> G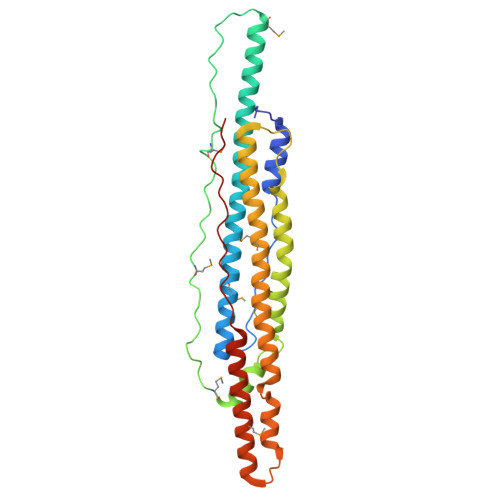SHMSEELQYELPGLERKAHECESTRPEGPGDATKPDELATTASVYSKLMASAAKLKATFAAGDREGERIAAAIRAAAGAYQKIEEQKAAELSRQMNGSDAPPPAAEAVVPDMSGIPGPLAIPSMEYPSAAAAADEMDWEAAARIIHSGDTQALSMKYFRDQWRDYQSTLEGHGRHFANPAEGWAGAAAETCAEAQRRLSTWWADMGAECGRLAQEATTFVDAHDKLVANHPTLENVREFEETEWASEWDRQNAWAMLQEQSEDALEAYANGSQIQEIRPGKPPSIGGLPI>[2x]MTQNVVIIDTGCANISSVKFAIERLGYAVTISRDPQVVLAADKLFLPGVGTASEAMKNLTERDLIELVKRVEKPLLGICL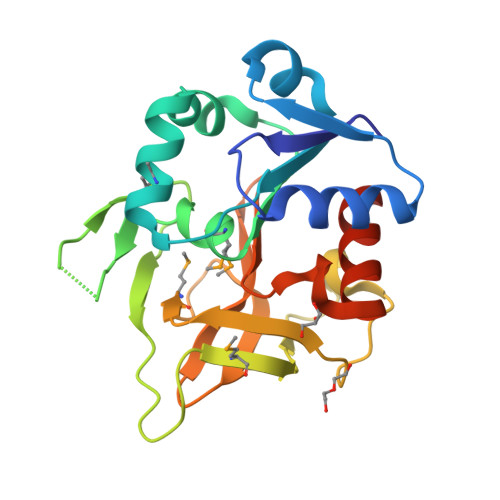GMQLLGKLSEEKGQKADEIVQCLGLVDGEVRLLQTGDLPLPHMGWNTVQVKEGHPLFNGIEPDAYFYFVHSFAMPVGDYTIAQCEYGQPFSAAIQAGNYYGVQFHPERSSKAGARLIQNFLELRGENLYFQ>[2x]GGGCCNGUCGUCUAXCCUGGUUAGGACGCCGCCCUUACAAG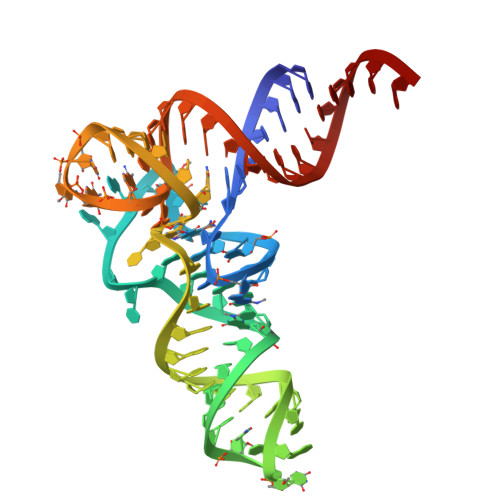GCGGAGGUCCUGGGUUCGAGUCCCAGCGGGCCCACCA>NIEVLNLVTGPDSITTIELYLNTRMGQNDESKDNYGYSEKVTVANSSDQDKPTSGEIPTYSTARINLPMLNEDLTSNTLTMWEAVSVKTEVVGVSSLVNVHMATKRMYDDKGIGFPVEGMNFHMFAVGGEPLELQFLTGNYRTDYSANDKLVVPPIKHQSTQGLNPHYKQKLTKDGAFPVECWCPDPSKNENTRYYGSYTGGQSTPPVLQFTNTVTTVLLDENGVGPLCKGDGLYVSCCDIV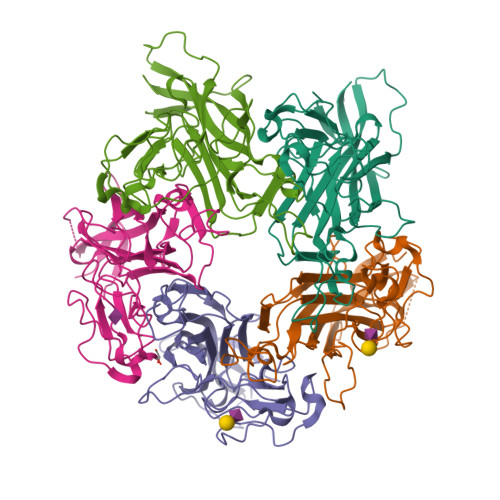GFLVGKDGDMQYRGLPRYFNILLRKRTVRN[10x]> SNIQQYKKTLSSITSD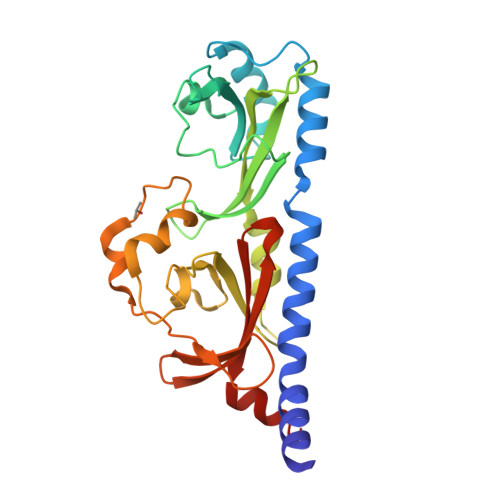LRENALFKAHTLQQTIPLNIDILALFSEIFDLDRGVPAEPDLALSKEMEKIFHSTYKEISLVKKEADGNFRVVASSRIEQLGKNYNQEIFLSDSQPFLATLRHSGSDSQVLAVLQTNIFDISSQEVLGVLYTLSDTNYLLNGLLAAKDPLSVKTAILSKNGIILQATDSSLDLVSIHKTVSKEQFCDVFLRDDICPPHLLLRPPLNLDPLPYGENFVSFCIGNTEMWGYIHSLPEMDFRILTYEEKSIIFASLWRR> GSHM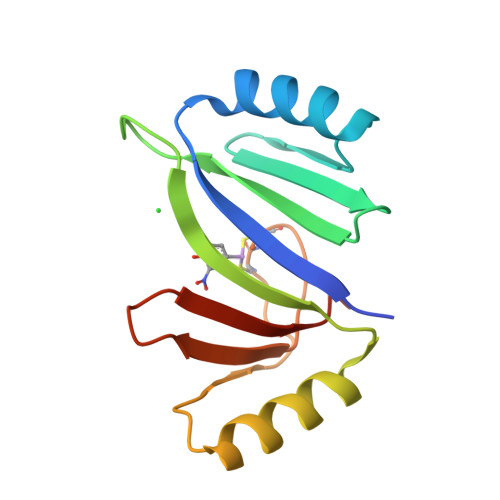SRVQLALRVPDLEASIGFYSKLFGTGPAKVRPGYANFAIAEPPLKLVLIEGAGEDATRLDHLGVEVEDSAQVGHAARRLKESGLATVEENDTACCYAVQDAVWVTGPGGEPWEVYVVKGDAD>[2x]MGS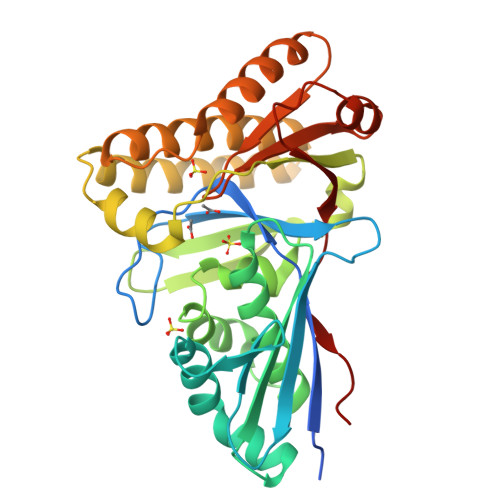SHHHHHHSSGLVPRGSMTYRSIGSTAYPTIGVVLLGGIANPVTRTPLHTSAGIAYSDSCGSIRSETRIYADEATHIYFNGTESTDDNRSVRRVLDRYSSVFEEAFGTKTVSYSSQNFGILSGSSDAGAASIGAAILGLKPDLDPHDVENDLRAVSESAGRSLFGGLTITWSDGFHAYTEKILDPEAFSGYSIVAFAFDYQRNPSDVIHQNIVRSDLYPARKKHADEHAHMIKEYAKTNDIKGIFDLAQEDTEEYHSILRGVGVNVIRENMQKLISYLKLIRKDYWNAYIVTGGSNVYVAVESENADRLFSIENTFGSKKKMLRIVGGAWHRRPE> YLDLF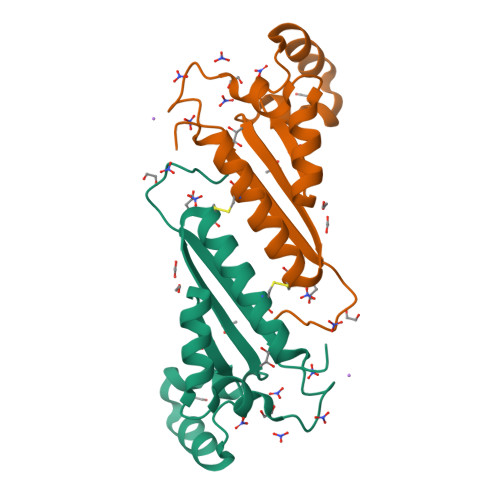SHKNMKLKERVLIPVKQYPKFNFVGKILGPQGNTIKRLQEETGAKISVLGKGSMRDKAKEEELRKGGDPKYAHLNMDLHVFIEVFGPPCEAYALMAHAMCEVKKFLVPDM> MNTKYNKEFLLYLAGFVDGDGSIIAQIEPNASYKFKHRLKLTFKVTQKTQRRWFLDKLVDEIGVGYVRDEGSVSNYILSEIKPLRNFLTQLQPFLKLKQKQANLVLKITEQLPSAKESPDKFLEVCTWVDQIAALNDSKTRKTTSETVRAV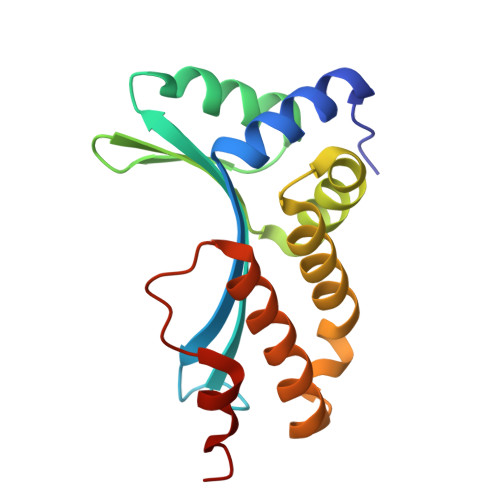LD> MAVPETRPNHTIYINNLNEKIKK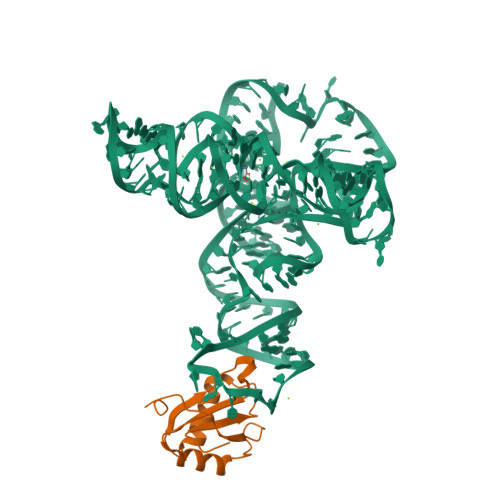DELKKSLHAIFSRFGQILDILVSRSLKMRGQAFVIFKEVSSATNALRSMQGFPFYDKPMRIQYAKTDSDIIAKMK> PLGSAMRELLLSDEYAEQKRAVNRFMLLLSTLYSLDAQAFAEATESLHGRTRVY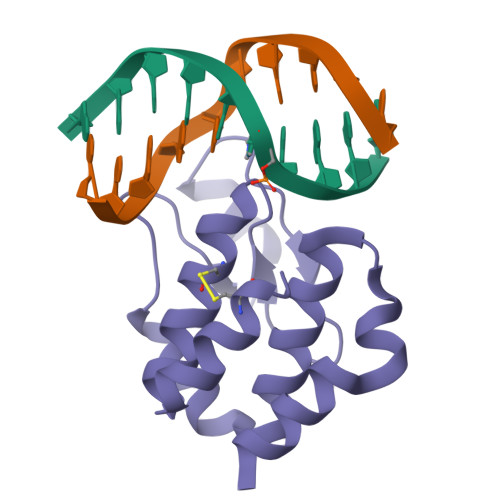FAADEQTLLKNGNQTKPKHVPGTPYWVITNTNTGRKCSMIEHIMQSMQFPAELIEKVCGTI>[8x]MKIAVLSRNPRLYSTRRLVEAGRERGHEMVVIDTLRAYMNIASHKPQIHYRGQPLEGFDAVIPRIGASVTFYGCAVLRQFEMMGVFPLNESVAIARSRDKLRSLQLLSRKGIGLPVTGFAHSPDDVPDLIEMVGGAPLVIKLLEGTQGIGVVLCETEKAAESVLEAFMGLKHNIMVQEYIKEAGGADIRCFVVGDKVIASMKRQAAPGEFRSNLHRGGSASLIKITPEERMTAIRAARVMGLNVAGVDILRSNHGPLVMEVNSSPGLEGIESTTGKDIAGIIIQYLEKNGGPHLARTKGKGKLAAALEHHHHHH;>[8x]EEEEEEEEEEEEEEEEEEEEEEEEEEEEEEEEEEEEEEEEEEEEEEEEEEEEEEEEEEEE

The RimK system allows for Pseudomonas spp. to adapt through post‐transcriptional regulation by altering the ribosomal subunit RpsF. RimK belongs to the ATP‐dependent carboxylate‐amine ligase superfamily of enzymes 13 , 24 which includes other members which can add amino acids to the C‐terminus of their target proteins. Each individual RimK unit has a classical ATP‐grasp fold with an elongated shape of approximately 60 x 35 x 30 Å. 25 The glutamate binding domain of each RimK subunit is linked to the ATP‐binding central domain by a flexible linker region, which is likely to allow the protein a range of motion to enable it to act like a classical “clam shaped” enzyme.

RimKPA was crystalized in the absence of its substrates; ATP, cdG, and glutamate whereas RimKPS was crystalized with both ATP and cdG present in the cryoprotectant. ADP and glutamate, of presumed cellular origin, were resolved in the RimKPA structure whereas ADP alone was resolved in the RimKPS structure. RimKPA has a slightly more closed tertiary structure in the center of the protein, leading to a more occluded active site that contains the predicted glutamate binding pocket. This occlusion is due to several factors, including the addition of a small section of β‐sheet in the core of the protein as well as the divergence of H2. In this study, we were able to resolve a peptide fitting the profile of poly‐α‐glutamate chains of either three or five amino acids long, in the active sites of seven out of eight of RimKPA monomer subunits. RimKPA chain A was examined in more detail as it was the most complete monomeric unit with a fully resolved structure as well as both ADP and glutamate bound. Interactions between side chains and residues less than 3 Å away were examined, confirming that the second resolved glutamate residue (E2) interacts with S68, E3 interacts with S7, R8 and R64, E4 interacts with S14 and finally E5 interacts with N262 and R189. 10 Intriguingly, a closer examination of the RimKPA structure highlighted a set of residues that were unresolved in several chains, and that correspond to the lower substrate binding loop. However, we observed significant differences between the ATPase activity of RimKPA and the other two Pseudomonas RimK homologs, with RimKPA showing a significantly reduced V max compared with both RimKPS and RimKPF. Conversely, the addition of increasing concentrations of RimBPA led to a reduction in RimKPA ATPase activity, suggesting that there are important, intrinsic differences between the responses of these two proteins to their corresponding binding partners.> GHMMNGDQNSDVYAQEKQDFVQHFSQIVRVLTEDEMGHPEIGDAIARLKEVLEYNAIGGKYNRGLTVVVAFRELVEPRKQDADSLQRAWTVGWCVELLQAFFLVADDIMDSSLTRRGQICWYQKPGVGLDAINDANLLEACIYRLLKLYCREQPYYLNLIELFLQSSYQTEIGQTLDLLTAPQGNVDLVRFTEKRYKSIVKYKTAFYSFYLPIAAAMYMAGIDGEKEHANAKKILLEMGEFFQ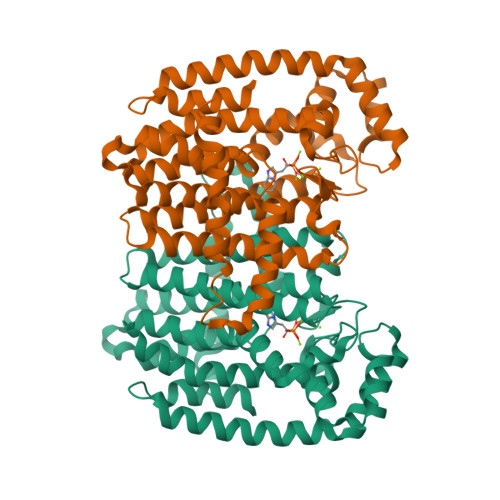IQDDYLDLFGDPSVTGKIGTDIQDNKCSWLVVQCLQRATPEQYQILKENYGQKEAEKVARVKALYEELDLPAVFLQYEEDSYSHIMALIEQYAAPLPPAVFLGLARKIYKRRK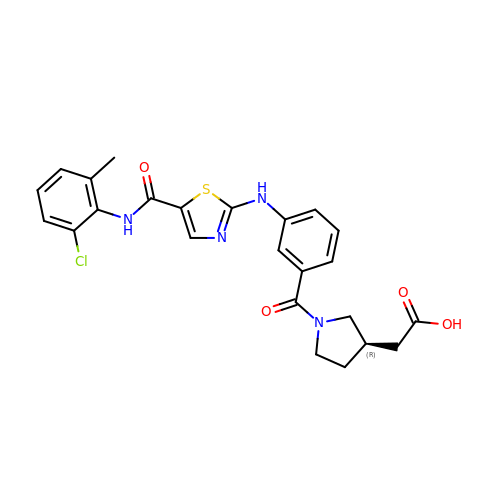2-[(3~{R})-1-[3-[[5-[(2-chloranyl-6-methyl-phenyl)carbamoyl]-1,3-thiazol-2-yl]amino]phenyl]carbonylpyrrolidin-3-yl]ethanoic acid | C24 H23 Cl N4 O4 S | VNOJDMNSDQAVOE-OAHLLOKOSA-N>DKLTLWTTPDPSPNCKIIEDKDSKLTLILTKCGSQILGSVSLLVVKGKFSNINNTTNPNEADKQITVKLLFDANGVLKQGSTMDSSYWNYRSDNSNLSQPYKKAVGFMPSKTAYPKQTKPTNKEISQAKNKIVSNVYLGGKIDQPCVIIISFNEEADSDYSIVFYFKWYKTYENVQFDSSSFNFSYIAQE[3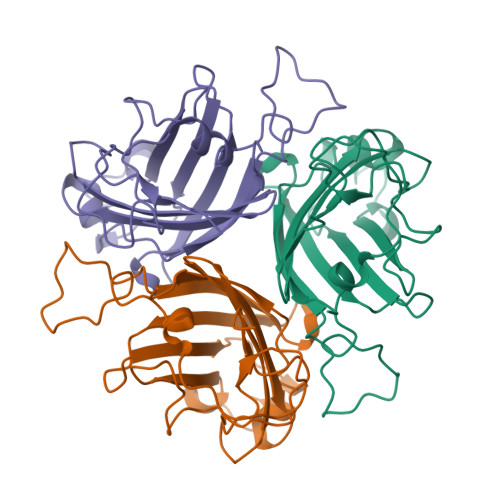x]>[2x]MADDQGCIEEQGVEDSANEDSVDAKPDRSSFVPSLFSKKKKNVTMRSIKTTRDRVPTYQYNMNFEKLGKCIIINNKNFDKVTGMGVRNGTDKDAEALFKCFRSLGFDVIVYNDCSCAKMQDLLKKASEEDHTNAACFA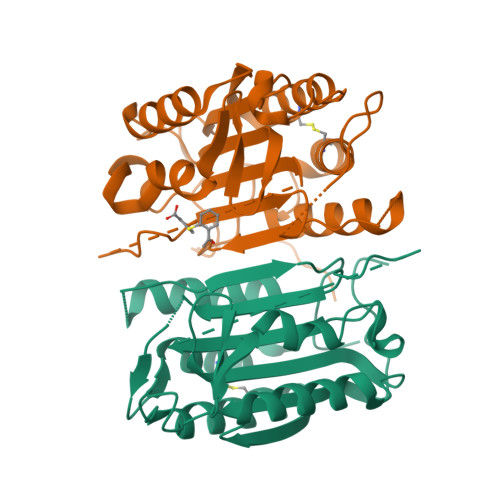CILLSHGEENVIYGKDGVTPIKDLTAHFRGDRCKTLLEKPKLFFIQACRGTELDDGIQADSGPINDTDANPRYKIPVEADFLFAYSTVPGYYSWRSPGRGSWFVQALCSILEEHGKDLEIMQILTRVNDRVARHFESQSDDPHFHEKKQIPCVVSMLTKELYFSQ> GGACCGCGG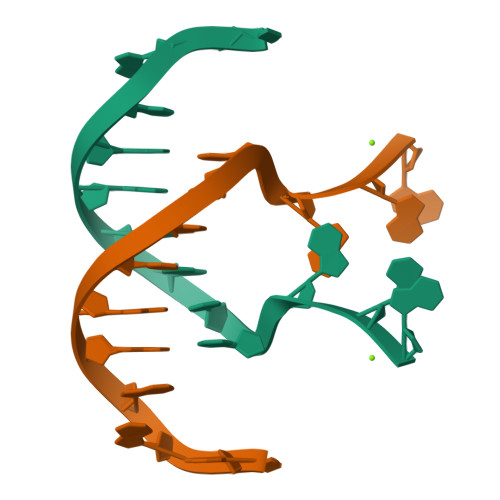GGAG>ETGCPANCLCSKTDINCKKPDDGNLFPLLEGQDSGSSNGQTSIQITDISRNITSIHIENWKNLQTLNAVDMELYTGLQRLTIRNSGLRNIQPRAFAKNPHLRYIDLSGNRLTTLSWQLFQTLRLFDLRLERNPFQCSCDIRWIQLWQEKGEANLQSQQLHCMNLDTAVILLRNMNITQCDLPEISVSHVNLTVREGENAVITCQGSGSPLPDVDWTVADLHSINTHQTNLQWTNVHAIQLTLVNVTSEDNGFLLTCIAENVVGMSQASVLLTVYGTKHHHHHH[3x];>ETGESPPVFIKKPVDQIG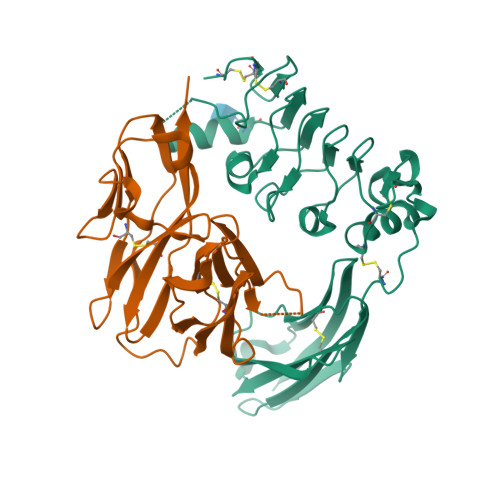VSGGVASFVCQATGDPKPRVTWNKKGKKVNSQRFETIEFDESAGAVLRIQPLRTPRDENIYECVAQNPHGEVTVHAKLTVLREDQLPPGFPNIDMGPQLKVVERTRTATMLCAASGNPDPEITWFKDFLPVDPSTSNGRIKQLRSGGLQIESSEETDQGKYECVASNSAGVRYSSPANLYVRVRRVAPRFSILPVSHEIMPGGNVNITCVAVGSPMPYVKWMQGAEDLTPEDDMPVGRNVLELTDVKDSANYTCVAMSSLGVIEAVAQITVKSKGHHHHHH[3x]>MRTYPVEIAGVRRELPIVQVGPGVAVALLNLLGDTELTEAAAEALAKRLPPEVEVLVTPEVKAVPLAHALSRITGKPYVVARKTEKPYMINPVSRQVLSITTGKP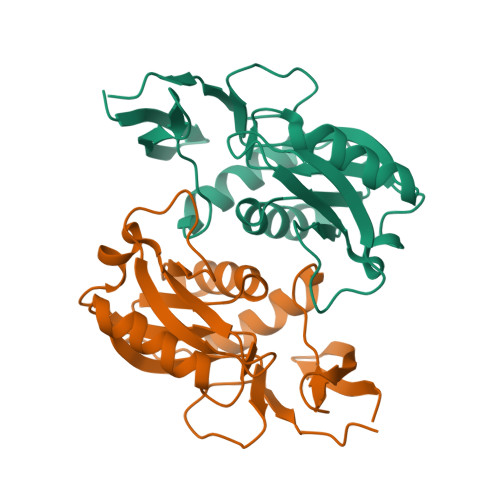QLLVLDGADIPRVRGKKVAIVDDVVSTGSTLAGLRELIESVGGEVVAVLAVFTEGTPRQDVVALGHLPLFKPE[6x]> DMRPEIWIAQEARRIGDE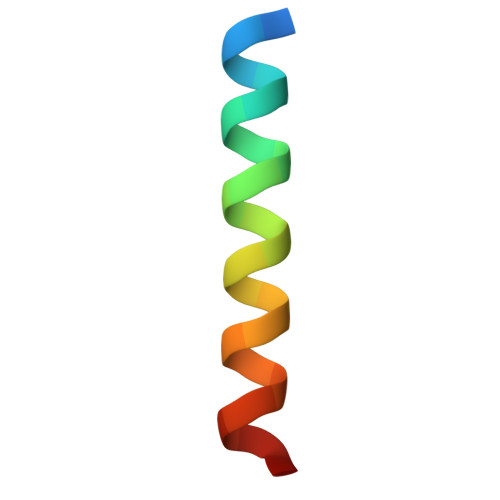ANAYYARR> MAAATADDEGSAATILKQAIAGDRSLVEAAEAISQQTLLRLACEVRQVGDRQPRFTATSIARVDVAPGCRLRFVLDGSPEDAYVTSEDYFKRCCGQSSYRGFAVAVLTANEDHVHSLAVPPLVLLHRFSLFNPRDLLDFELACLLMYLENCPRSHATPSTFAKVLAWLGVAGRRTSPFERVRCLFLRSCHWVLNTLMFMVHVKPFDDEFVLPHWYMARYLLANNPPPVLSALFCATPTSSSFRLPGPPPRSDCVAYNPAGIMGSCWASEEVRAPLVYWWLSETPKRQTSSLFYQFCGSLEVL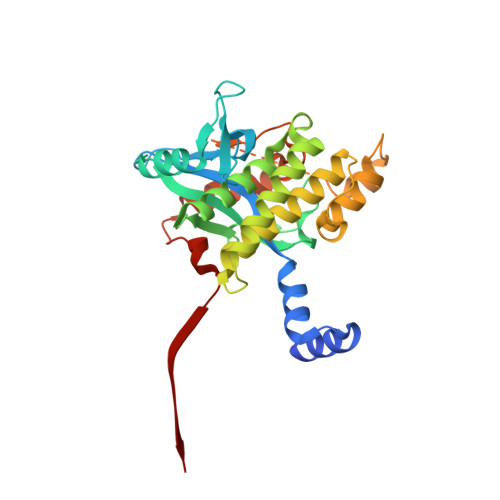FQ>[2x]PMILGYWNVRGLSHPIRLLLEYTDSSYEEKRYAMGDAPDYDRSQWLNEKFKLGLDFPNLPYLIDGSRKITQSNAIMRYLARKHHLCGETEEERIRADIVENQVMDNRMQL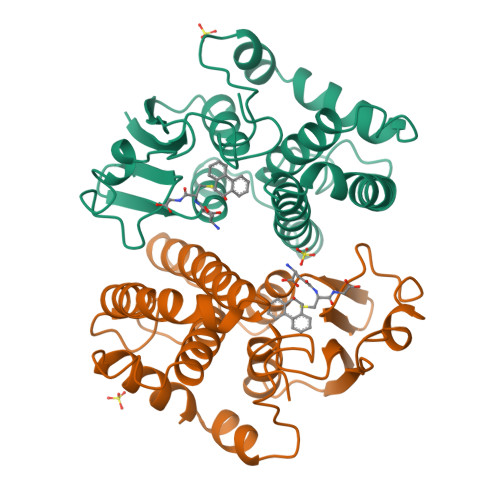IMLCYNPDFEKQKPEFLKTIPEKMKLYSEFLGKRPWFAGDKVTYVDFLAYDILDQYHIFEPKCLDAFPNLKDFLARFEGLKKISAYMKSSRYLSTPIFSKLAQWSNK>[4x]MGGSHHHHHHGMASLENLYFQADQPIDADVTVIGSGPGGYVAAIKAAQLGFKTVCIEKNETLGGTCLNVGCIPSKALLNNSHYYHMAHGKDFASRGIEMSEVRLNLDKMMEQKSTAVKALTGGI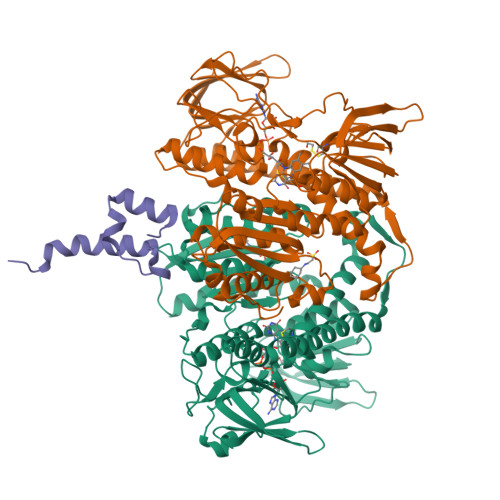AHLFKQNKVVHVNGYGKITGKNQVTATKADGGTQVIDTKNILIATGSEVTPFPGITIDEDTIVSSTGALSLKKVPEKMVVIGAGVIGVELGSVWQRLGADVTAVEFLGHVGGVGIDMEISKNFQRILQKQGFKFKLNTKVTGATKKSDGKIDVSIEAASGGKAEVITCDVLLVCIGRRPFTKNLGLEELGIELDPRGRIPVNTRFQTKIPNIYAIGDVVAGPMLAHKAEDEGIICVEGMAGGAVHIDYNCVPSVIYTHPEVAWVGKSEEQLKEEGIEYKVGKFPFAANSRAKTNADTDGMVKILGQKSTDRVLGAHILGPGAGEMVNEAALALEYGASCEDIARVCHAHPTLSEAFREANLAASFGKSINF;>GEIKGRKTLATPAVRNLAMENNIKLSEVVGSGKDGRILKEDILNYLEKQTLEHHHHHH[2x]> GSHMSEKEIRRSMPLFPIGPVMKLTDLTARQIRYYEDQGLIHPARNQGNHRLYSLQDIDVLLEIKDYLNDGLNIAGIKKMYQMQQ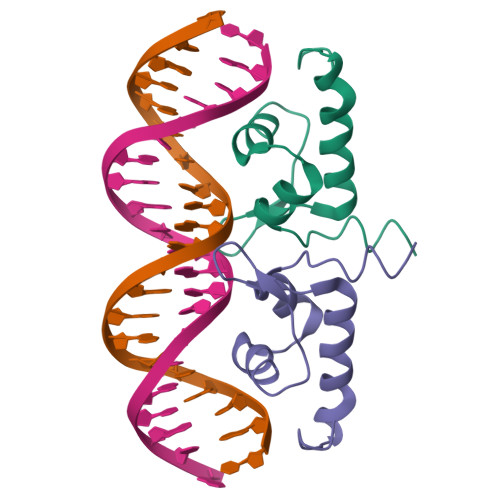KESKEPLTDDDVRKILRKEMQQAGRFVKQDATGKQQLPRF2'-(3-METHYL-4-DIMETHYLAMINOPHENYL)-5-(4-METHYL-1-PIPERAZINYL)-2,5'-BI-BENZIMIDAZOLE | C28 H31 N7 | 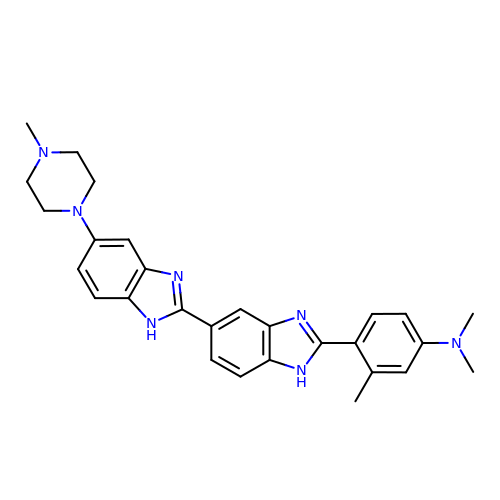ADKLMOJIJGHCCD-UHFFFAOYSA-N> MSVLRPLDKLPGLNTATILLVGTEDALLQQLADSMLKEDCASELKVHLAKSLPLPSSVNRPRIDLIVFVVNLHSKYSLQNTEESLRHVDASFFLGKVCFLATGAGRESHCSIHRHTVVKLAHTYQSPLLYCDLEVEG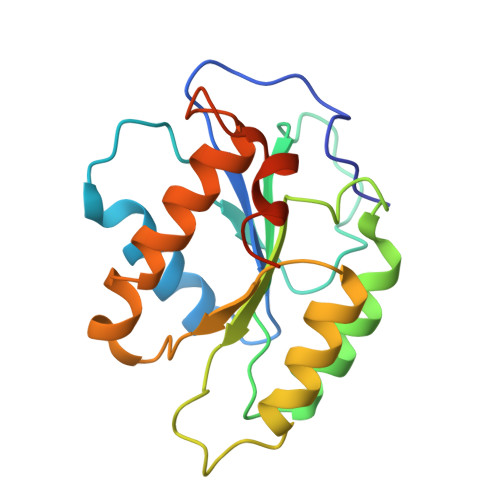FRATMAQRLVRVLQICAGHVPGVSALNLLSLLRSSEGPSLEDL>MAHAMENSWTISKEYHIDEEVGFALPNPQENLPDFYNDWMFIAKHLPDLIESGQLRERVEKLNMLSIDHLTDHKSQRLARLVLGCITMAYVWGKGHGDVRKVLPRNIAVPYCQLSKKLELPPILVYADCVLANWKKKDPNKPLTYENMDVLFSFRDGDCSKGFFLVSLLVEIAAASAIKVIPTVFKAMQMQERDTLLKALLEIASCLEKALQVFHQIHDHVNPKAFFSVLRIYLSGWKGNPQLSDGLVYEGFWEDPKEFAGGSAGQSSVFQCFDVLLGIQQTAGGGHAAQFLQDMRRYMPPAHRNFLCSLESNPSVREFVLSKGDAGLREAYDACVKALVSLRSYHLQIVTKYILIPASQQPKENKTSEDPSKLEAKGTGGTDLMN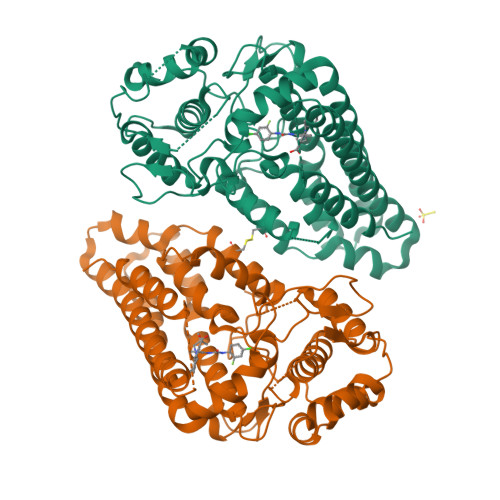FLKTVRSTTEKSLLKEG[2x]> MHSTLRVFTKNNCLSFTNMNRFSTAAQVAQANYSKFRADYSASVAAFQQRIKTIEKENTGSMKKPMAKAYEHPYNSEHHPLNFSAVKIAETFHDFIGPEQVSPHYESFAMSRKFLLTFWGGFFVLNFGMATVDLNWIMKSTYIPWIFWFQLMYFYVEGKNSMFMPLLQRFYRRAAANEIFTMEAFYHENIENKLRNLMRITKGQLEYWDIHTSYGEIRAD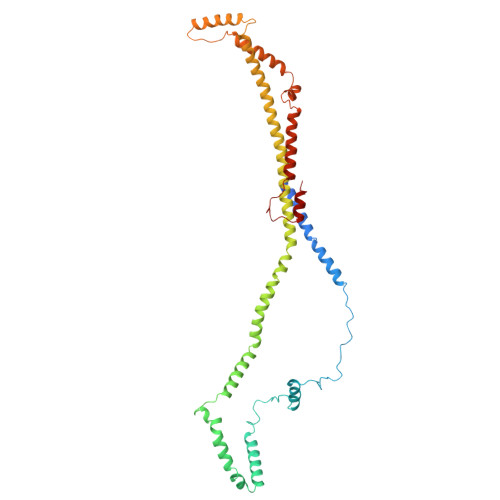SINNFLANEYLRLQSHITSRALNILKQAQAYETMNQAALLQKLIDDATSAIDNALKGDKKAEVLARSLDSAIDGLSKGYMDYQNDPLLPLILSSIEANVKKITTLSAQEQANLIGLTAEQLKSIKENDVRARKEFLESQPKLDNNLKNIESVKKILATWGK>[2x]MELWLVRHGETLWNREGRLLGWT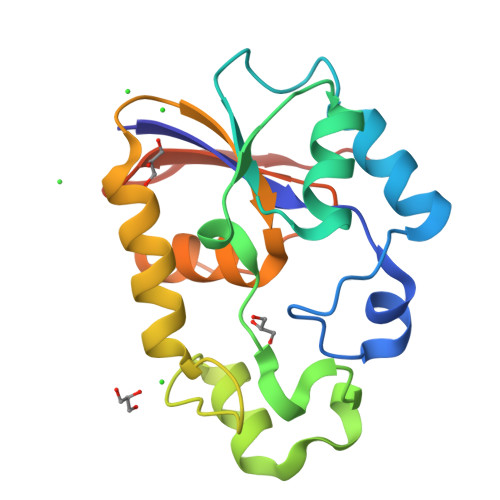DLPMTAEGEAQARRLKGALPSLPAFSSDLLRARRTAELAGFSPRLYPELREIHFGALEGALWETLDPRYKEALLRFQGFHPPGGESLSAFQERVFRFLEGLKAPAVLFTHGGVVRAVLRALGEDGLVPPGSAVAVDWPRRVLVRLALDGEEATG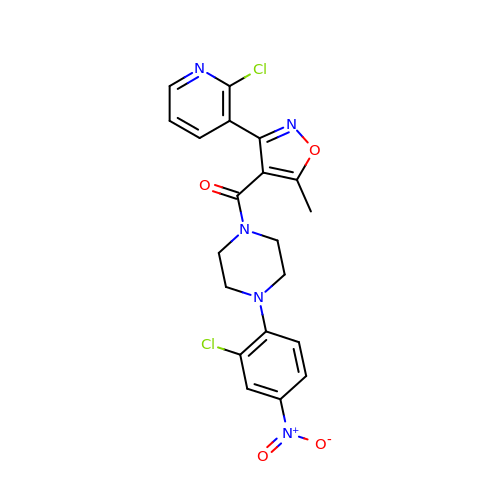[4-(2-chloro-4-nitrophenyl)piperazin-1-yl][3-(2-chloropyridin-3-yl)-5-methyl-1,2-oxazol-4-yl]methanone | C20 H17 Cl2 N5 O4 | OVZFTYKFOMVVNQ-UHFFFAOYSA-N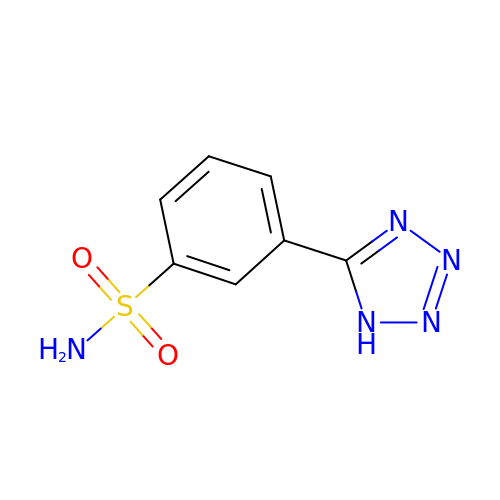5-(3-SULFAMOYLPHENYL)-1H-1,2,3,4-TETRAZOL-1-IDE | C7 H7 N5 O2 S | BIOBAIFFWOWFPU-UHFFFAOYSA-N>MALLAEHLLKPLPADKQIETGPFLEAVSHLPPFFDCLGSPVFTPIKADISGNITKIKAVYDTNPAKFRTLQNILEVEKEMYGAEWPKVGATLALMWLKRGLRFIQVFLQSICDGERDENHPNLIRVNATKAYEMALKKYHGWIVQKIFQAALYAAPYKS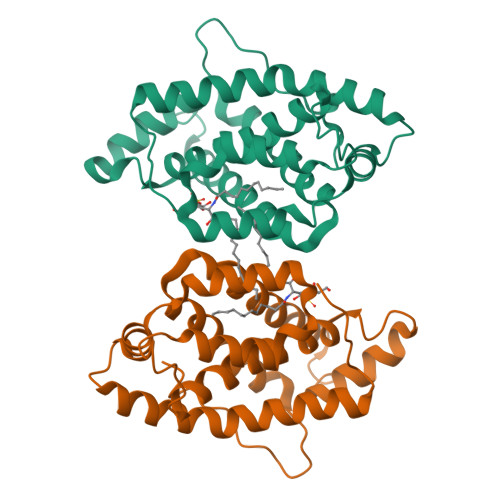DFLKALSKGQNVTEEECLEKIRLFLVNYTATIDVIYEMYTQMNAELNYKV[4x]> MNHKVHHHHHHMDIKKVYLKGQEEAKGWNKPNKIIIHHPEYNGSIEGLN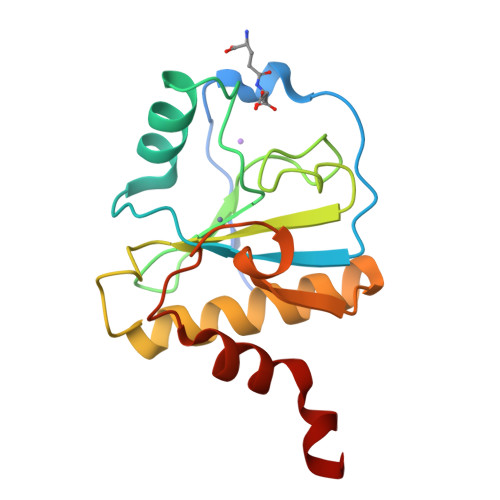DIMRSMGFYMIGYNFYVRKDGTVYEGRPVWATGANCYGHNHDSIGVCFEGNYDKETDMPQEQFNAGVELIKYLKSKYGINEVNGHKHYYNTACPGQYFPLEKMLSCLDGQLQQE> MLNKKLDKKDKDAYPVESEIINLTINGVARGNHFNFVNGTLQTRNYGKVYVAGQGTSDSELVKKKGDIILTSLLGDGDHTLNVNKAE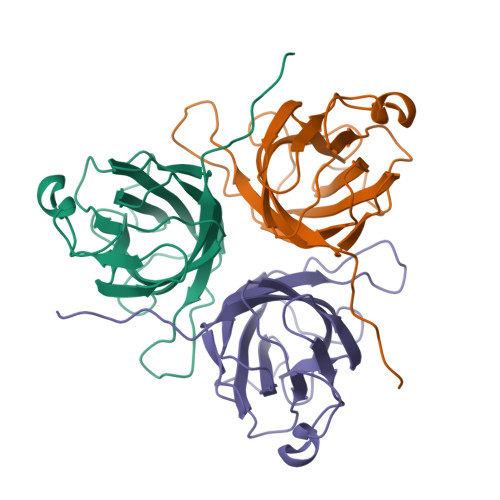SKELELYARVYNNTKRDITVDSVSLSPGLNATGREFSANKFVLYFKPTVLKKNRINTLVFGATFDEDIDDTNRHYLLSMRFSPGNDLFKVGEKLEHHHHHH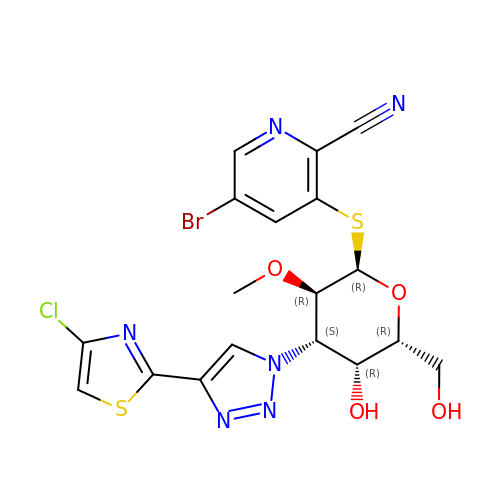5-bromanyl-3-[(2~{R},3~{R},4~{S},5~{R},6~{R})-4-[4-(4-chloranyl-1,3-thiazol-2-yl)-1,2,3-triazol-1-yl]-6-(hydroxymethyl)-3-methoxy-5-oxidanyl-oxan-2-yl]sulfanyl-pyridine-2-carbonitrile | C18 H16 Br Cl N6 O4 S2 | MZSZXCMHHUHYMW-PTERYMMESA-N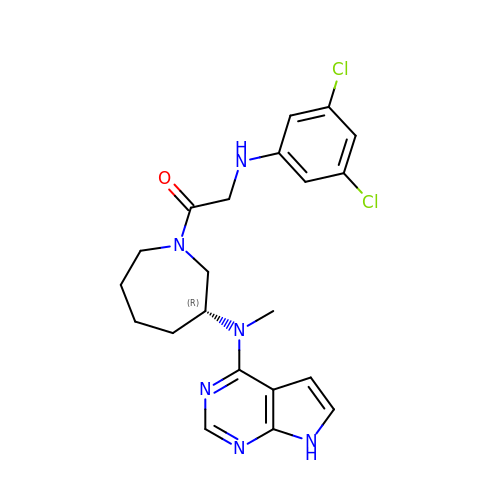2-(3,5-dichloroanilino)-1-{(3R)-3-[methyl(7H-pyrrolo[2,3-d]pyrimidin-4-yl)amino]azepan-1-yl}ethan-1-one | C21 H24 Cl2 N6 O | OGVYBLOWEVEGIK-QGZVFWFLSA-N>[2x]HHHHHHSSGLVPRGSHMISKEYHIDEEVGFALPNPQENLPDFYNDWMFIAKHLPDLIESGQLRERVEKLNMLSIDHLTDHKSQRLARLVLGCITMAYVWGKGHGDVRKVLPRNIAVPYCQLSKKLEL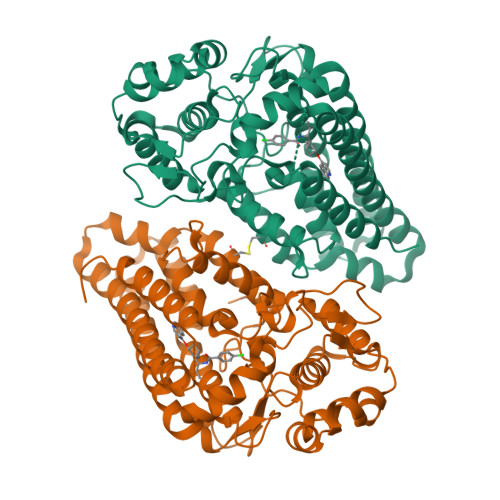PPILVYADCVLANWKKKDPNKPLTYENMDVLFSFRDGDCSKGFFLVSLLVEIAAASAIKVIPTVFKAMQMQERDTLLKALLEIASCLEKALQVFHQIHDHVNPKAFFSVLRIYLSGWKGNPQLSDGLVYEGFWEDPKEFAGGSAGQSSVFQCFDVLLGIQQTAGGGHAAQFLQDMRRYMPPAHRNFLCSLESNPSVREFVLSKGDAGLREAYDACVKALVSLRSYHLQIVTKYILIPASQQPKENKTSEDPSKLEAKGTGGTDLMNFLKTVRSTTEKSLLKEG> GPDSMSLLEQLARKRIEKSKGLLSADQSHSTSKSASLLERLHKNRETKDNNAETKRKDLKTLLAKDKVKRSDFTPNQHSVSLSLKLSALKKSNSDLEKQGKSVTLDSKENELPTKRKSPDDKL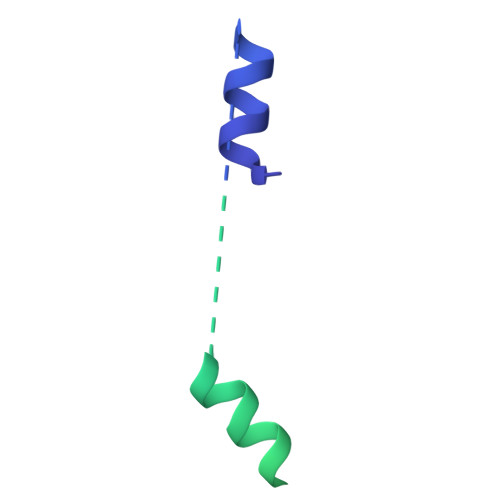NLEESWKAIKEMNHYCFLKNDPCINQTDDFAFTNFIIKDKKNSLSTSIPLSSQNSSFLSLKKHNNELLGIFVPCNLPKTTRKVAIENFNRPSPDDIIQSAQLNAFNEKLENLNIKSAGSWSHPQFEK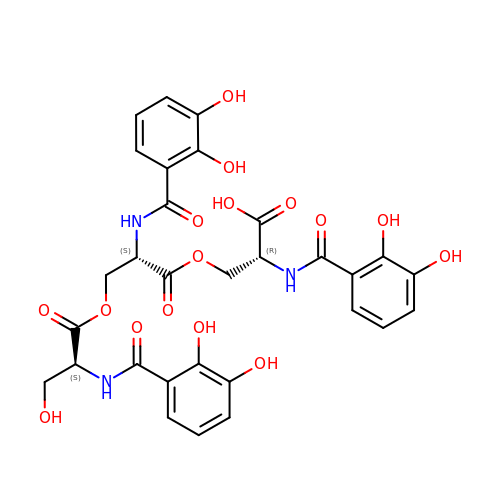N-[(2,3-dihydroxyphenyl)carbonyl]-O-[(2S)-2-{[(2,3-dihydroxyphenyl)carbonyl]amino}-3-({N-[(2,3-dihydroxyphenyl)carbonyl]-L-seryl}oxy)propanoyl]-D-serine | C30 H29 N3 O16 | NTWRWGRCGVKQNS-KSZLIROESA-N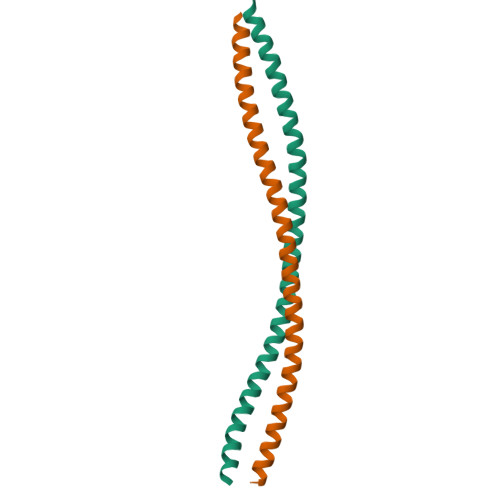>GPGSDEAAALRAELRDLELEEARLVQELEDVDRNNARAAADLQAAQAEAAELDQQERQHYRDYSALKRQQLELLDQLGNVENQLQYARVQLDRLKE[4x]> GAACGACACAGA;> CGG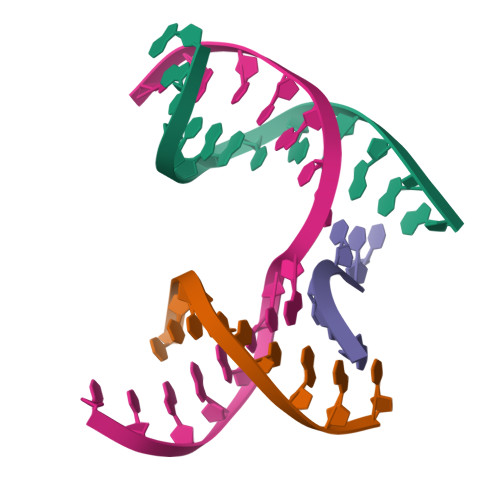TGACTC;> TCTCCG;> TCGAGTCAGTGTCGT>AEPVYPDQLRLFSLGQGVCGDKYRPVNREEAQSVKSNIVGMMGQWQISGLANGWVIMGPGYNGEIKPGTASNTWCYPTNPVTGEIPTLSALDIPDGDEVDVQWRLVHDSANFIKPTSYLAHYLGYAWVGGNDSQYVGEDMDVTRDGDGWVIRGNNDGGCDGYRCGDKTAIKVSNFAYNLDPDSFKHGDVTQSDRQLVKTVVGWAVNDSDTPQSGYDVTLRYDTATNWSKTNTYGLSEKVTTKNKFKWPLVGETELSIEIAANQSWASQNGGSTTTSLSQSVRPTVPARSKIPVKIELYKADISYPYEFKADVSYDLTLSGFLRWGGNAWYTHPDNRPNWNHTFVIGPYKDKASSIRYQWDKRYIPGEVKWWDWNWTIQQNGL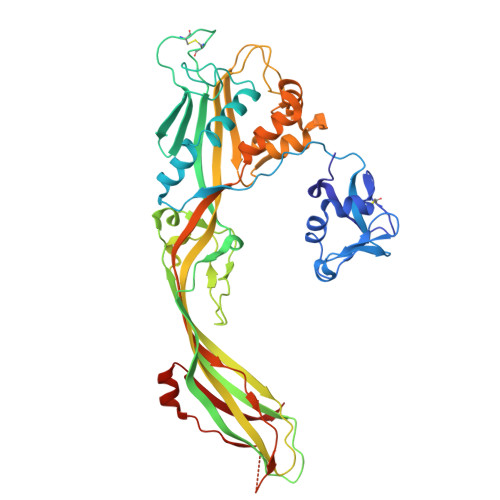STMQNNLARVLRPVRAGITGDFSAESQFAGNIEIGAPVPLAADSKVRRARSVDGAGQGLRLEIPLDAQELSGLGFNNVSLSVTPAANQ[2x]> MKIYRPLWEDGAFLMPQQFQQQAAWDVHLADSVARMGLAHPWGVVAAEFDDSLLPLSRLNATRLIVRFPDGTLIDTERADNLPPVCDLSTVSDRSLVDIVLALPLLNANGGNLDNGSESERPRRWKSERVNVQELAGHEQSEVAVLRHNLTLRMAHQENAAWLTCPVTRLVRDAQGQWCRDPRFIPPLL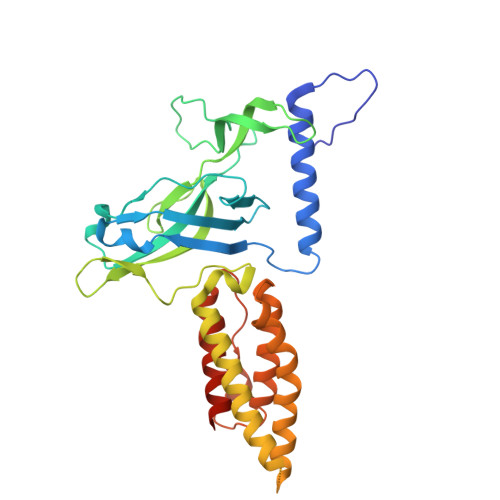TLSASPSLMTELAELLHHLQARRQRLMSMRRENNARLADFAVADVSLFWLLNALNSAEPVLKELLDMPYRHPELLYRELARLAGSLLTFSLEHNVDAVPAYHHETPENVFPPLLSLLNRLLEASLPSHHHHHH>EQTYYDLVKAFMAEIRQYIRELNLIIKVFREPFVSNSKLFSANDVENIFSRIVDIHELSVKLLGHIEDTVEMTDEGSPHPLVGSCFEDLAEELAFDPYESYARDILRPGFHDRFLSQLSKPGAALYLQSIGEGFKEAVQYVLPRLLLAPVYHCLHYFELLKQLEEKSEDQEDKECLKQAITALLNVQSGMEKICSKSLAKRRLSESACRFYSQQMKGKQLAIKKMNEIQKNIDGWEGKDIGQCCNEFIMEGTLTRVGAKHERHIFLFDGLMICCKSNHGQPRLPGASNAEYRLKEKFFMRKVQINDKDDTNEYKHAFEIILKDENSVIFSAKSAEEKNNWMAALISLQYRSTLERMLDVTMLQEEKEEQMRLPSADVYRFAEPDSEENIIFEENMQPKAGIPIIKAGTVIKLIERLTYHMYADPNFVRTFLTTYRSFCKPQELLSLIIERFEIPEPEPTEADRIAIENGDQPLSAELKRFRKEYIQPVQLRVLNVCRHWVEHHFYDFERDAYLLQRMEEFIGTVRGKAMKKWVESITKIIQRKKIARDNGPGHNITFQSSPPTVEWHISRPGHIETFDLLTLHPIEIARQLTLLESDLYRAVQPSELVGSVWTKEDKEINSPNLLKMIRHTTNLTLWFEKC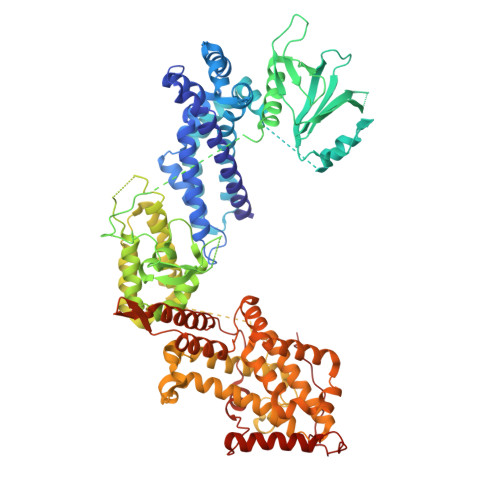IVETENLEERVAVVSRIIEILQVFQELNNFNGVLEVVSAMNSSPVYRLDHTFEQIPSRQKKILEEAHELSEDHYKKYLAKLRSINPPCVPFFGIYLTNILKTEEGNPEVLKRHGKELINFSKRRKVAEITGEIQQYQNQPYCLRVESDIKRFFENLNPMGNSMEKEFTDYLFNKSLEIEPRNPKPLPRFPKKYSYPLKSPGVRPSN[2x]> MSGSHHHHHHSSGIEGRGRLIKHMTAEAGITGTWYNQLGSTLIVTAGADGALTGTYESAVGNAESSYVLTGRYDS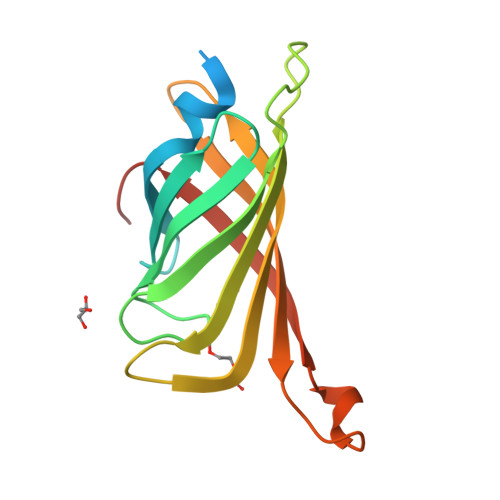APATDGSGTALGWTVAWKNNYRNAHSASTWSGQYVGGAEARINTQVLTTSGTTEANAWKSTLVGHDTFTKVKPSAASI> MKWCSTYIIIWLAIIFHKFQKSTATASHNIDDILQLKDDTGVITVTADNYPLLSRGVPGYFNILYITMRGTNSNGMSCQLCHDFEKTYHAVADVIRSQAPQSLNLFFTVDVNEVPQLVKDLKLQNVPHLVVYPPAESNKQSQFEWKTSPFYQYSLVPENAENTLQFGDFLAKILNISITVPQAFNVQEFVYYFVACMVVFIFI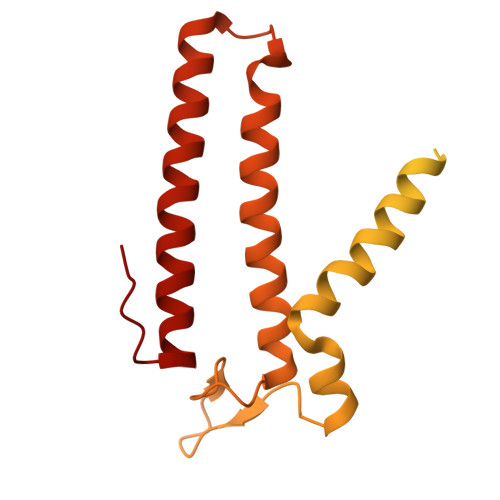KKVILPKVTNKWKLFSMILSLGILLPSITGYKFVEMNAIPFIARDAKNRIMYFSGGSGWQFGIEIFSVSLMYIVMSALSVLLIYVPKISCVSEKMRGLLSSFLACVLFYFFSYFISCYLIKNPGYPIVF2-phenylazanyl-9~{H}-purine-6-carbonitrile 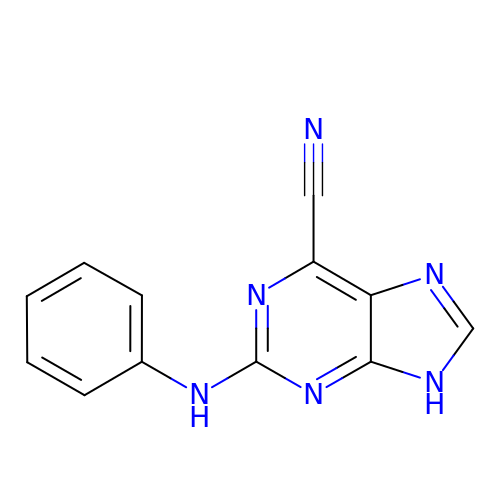| C12 H8 N6 | CVPBLNRTHSCHMF-UHFFFAOYSA-N alpha-D-arabinopyranose | C5 H10 O5 | 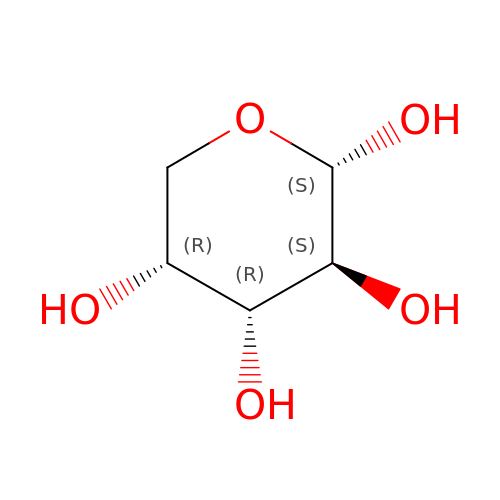SRBFZHDQGSBBOR-MBMOQRBOSA-N> SPSVEACGYSDRVAQLTVGNSSITTQEAANIVLAYGEWPEYCPDTDATAVDKPTRPDVSVNRFYTLDSKMWQENSTGWYWKFPDVLNKTGVFGQNAQFHYLYRSGFCLHVQCNASKFHQGALLVAVIPEFVIAGRGSNTKPNEAPHPGFTTTFPGTTGATFYDPYVLDSGVPLSQALIYPHQWINLRTNNCATVIVPYINAVPFDSAINHSNFGLIVI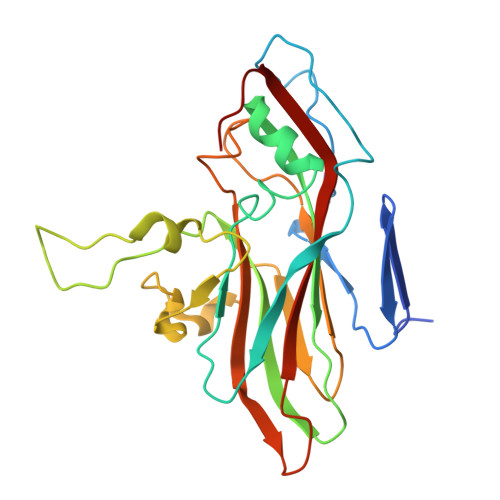PVSPLKYSSGATTAIPITITIAPLNSEFGGLRQAVSQ> TETTSFSITKFGPDQQNLIFQGDGYTTKERLTLTKAVRNTVGRALYSSPIHIWDSKTGNVANFVTSFTFVIDAPNSYNVADGFTFFIAPVDTKPQTGGGYLGVFNSKDYDKTSQ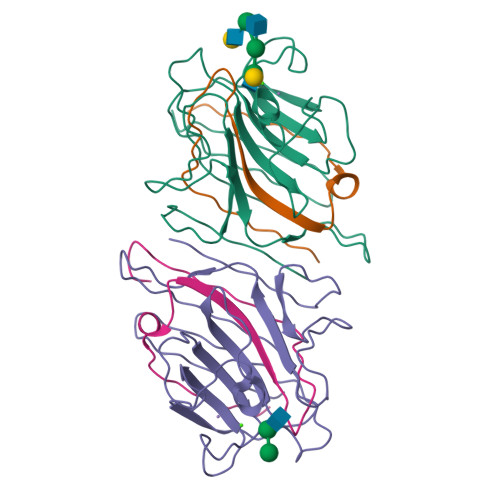TVAVEFDTFYNTAWDPSNGDRHIGIDVNSIKSINTKSWALQNGKEANVVIAFNAATNVLTVSLTYPN;> ETSYTLNEVVPLKEFVPEWVRIGFSATTGAEFAAHEVLSWYFHSELAGTSSS;> TETTSFSITKFGPDQQNLIFQGDGYTTKERLTLTKAVRNTVGRALYSSPIHIWDSKTGNVANFVTSFTFVIDAPNSYNVADGFTFFIAPVDTKPQTGGGYLGVFNSKDYDKTSQTVAVEFDTFYNTAWDPSNGDRHIGIDVNSIKSINTKSWKLQNGKEANVVIAFNAATNVLTVSLTYPN;> ETSYTLNEVVPLKEFVPEWVRIGFSATTGAEFAAHEVLSWYFHSELAGTSSN>[2x]GSM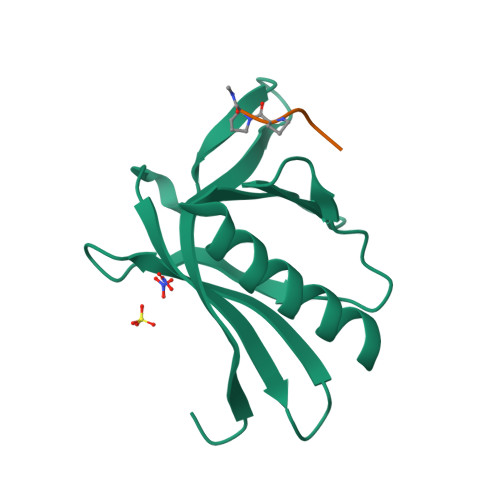SEQSICQARAAVMVYDDANKKWVPAGGSTGFSRVHIYHHTGNNTFRVVGRKIQDHQVVINCAIPKGLKYNQATQTFHQWRDARQVYGLNFGSKEDANVFASAMMHALEVL N-({(2E)-2-[(4-nitrophenyl)methylidene]hydrazino}carbonothioyl)-beta-D-glucopyranosylamine | C14 H18 N4 O7 S | 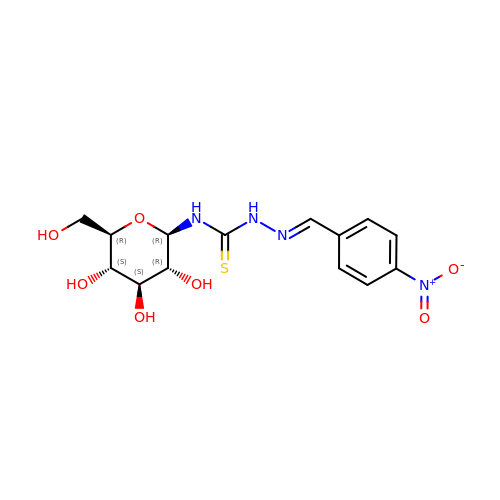GUSXRMQWONZMDY-IVSPNHRTSA-N>MAKEYKTITQIAGPLIFVEKTEPVGYNEIVNIKMGDGTVRRGQVLDSSADIVVVQVFEGTGGLDKDCGVIFTGETLKLPASVDLLGRILSGSGEPRDGGPRIVPDQLLDINGAAMNPYARLPPKDFIQTGISTIDGTNTLVRGQKLPIFSASGLPHTEIALQIARQASVPGSESAFAVVFAAMGITNEEAQYFMSDFEKTGALERAVVFLNLADDPAVERIVTPRMALTAAEYLAYEHGMHVLVILTDITNYAEALRQMGAARNEVPGRRGYPGYMYTDLATLYERAGIVKGAKGSV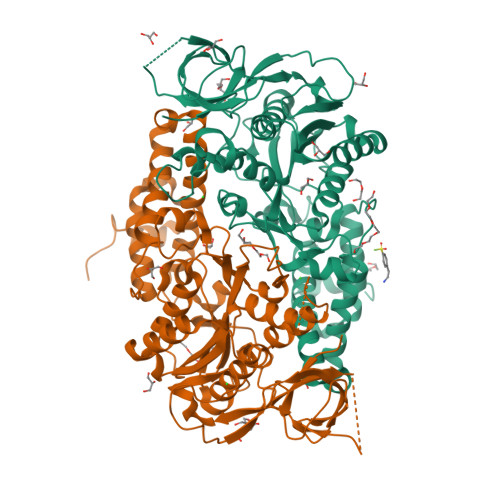TQIPILSMPGDDITHPIPDLSGYITEGQIVVARELHRKGIYPPINVLPSLSRLMNSGIGAGKTREDHKAVSDQMYAGYAEGRDLRGLVAIVGKEALSERDTKFLEFADLFEDKFVRQGRNENRTIEDTLEIGWQILTHLPENQLGRIDNKYIQKYHPAHRKAK[2x]>[4x]MSQHNEKNPHQHQSPLHDSSEAKPGMDSLAPEDGSHRPAAEPTPPGAQPTAPGSLKAPDTRNEKLNSLEDVRKGSENYALTTNQGVRIADDQNSLRAGSRGPTLLEDFILREKITHFDHERIPERIVHARGSAAHGYFQPYKSLSDITKADFLSDPNKITPVFVRFSTVQGGAGSADTVRDIRGFATKFYTEEGIF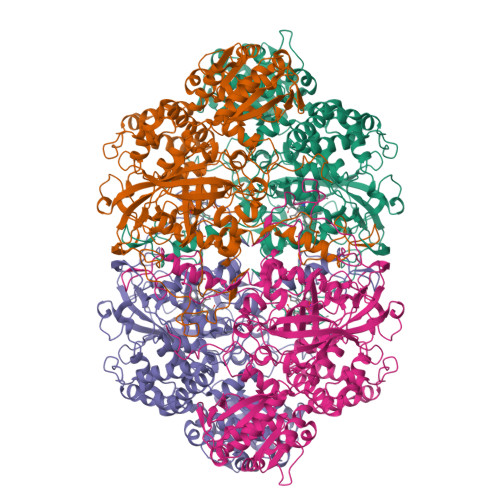DLVGNNTPIFFIQDAHKFPDFVHAVKPEPHWAIPQGQSAHDTFWDYVSLQPETLHNVMWAMSDRGIPRSYRTMEGFGIHTFRLINAEGKATFVRFHWKPLAGKASLVWDEAQKLTGRDPDFHRRELWEAIEAGDFPEYELGFQLIPEEDEFKFDFDLLDPTKLIPEELVPVQRVGKMVLNRNPDNFFAENEQAAFHPGHIVPGLDFTNDPLLQGRLFSYTDTQISRLGGPNFHEIPINRPTCPYHNFQRDGMHRMGIDTNPANYEPNSINDNWPRETPPGPKRGGFESYQERVEGNKVRERSPSFGEYYSHPRLFWLSQTPFEQRHIVDGFSFELSKVVRPYIRERVVDQLAHIDLTLAQAVAKNLGIELTDDQLNITPPPDVNGLKKDPSLSLYAIPDGDVKGRVVAILLNDEVRSADLLAILKALKAKGVHAKLLYSRMGEVTADDGTVLPIAATFAGAPSLTVDAVIVPCGNIADIADNGDANYYLMEAYKHLKPIALAGDARKFKATIKIADQGEEGIVEADSADGSFMDELLTLMAAHRVWSRIPKIDKIPA>[2x]HHHHHHLESTSLYKKAGMATANGAVENGQPDRKPPALPRPIRNLEVKFTKIFINNEWHESKSGKKFATCNPSTREQICEVEEGDKPDVDKAVEAAQVAFQRGSPWRRLDALSRGRLLHQLADLVERDRATLAALETMDTGKPFLHAFFIDLEGCIRTLRYFAGWADKIQGKTIPTDDNVVCFTRHEPIGVCGAITPWNFPLLMLVWKLAPALCCGNTMVLKPAEQTPLTALYLGSLIKEAGFPPGVVNIVPGFGPTVGAAISSHPQINKIAFTGSTEVGKLVKEAASRSNLKRVTLELGGKNPCIVCADADLDLAVEC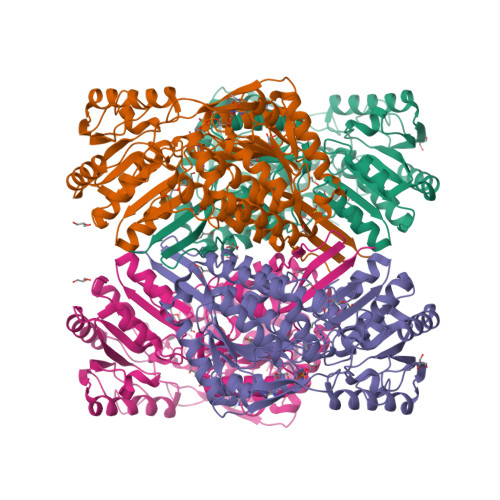AHQGVFFNQGQCCTAASRVFVEEQVYSEFVRRSVEYAKKRPVGDPFDVKTEQGPQIDQKQFDKILELIESGKKEGAKLECGGSAMEDKGLFIKPTVFSEVTDNMRIAKEEIFGPVQPILKFKSIEEVIKRANSTDYGLTAAVFTKNLDKALKLASALESGTVWINCYNALYAQAPFGGFKMSGNGRELGEYALAEYTEVKTVTIKLGDKNP> DYKDDDDKSHSPHLPRPHSRVPPHPSSERRAVYIGALFPMSGGWPGGQACQPAVEMALEDVNSRRDILPDYELKLIHHDSKCDPGQATKYLYELLYNDPIKIILMPGCSSVSTLVAEAARMWNLIVLSYGSSSPALSNRQRFPTFFRTHPSATLHNPTRVKLFEKWGWKKIATIQQTTEVFTSTLDDLEERVKEAGIEITFRQSFFSDPAVPVKNLKRQDARIIVGLFYETEARKVFCEVYKERLFGKKYVWFLIGWYADNWFKIYDPSINCTVDEMTEAVEGHITTEIVMLNPANTRSISNMTSQEFVEKLTKRLKRHPEETGGFQEAPLAYDAIWALALALNKTSGGGGRSGVRLEDFNYNNQTITDQIYRAMNSSSFEGVSGHVVFDASGSRMAWTLIEQLQGGSYKKIGYYDSTKDDLSWSKTDKWIGGSPPADQTLVIKTFRFLSQKLFISVSVLSSLGIVLAVVCLSFNIYNSHVRYIQNSQPNLNNLTAVGCSLALAAVFPLGLDGYHIGRNQFPFVCQARLWLLGLGFSLGYGSMFTKIWWVHTVFTKKEEKKEWRKTLEPWK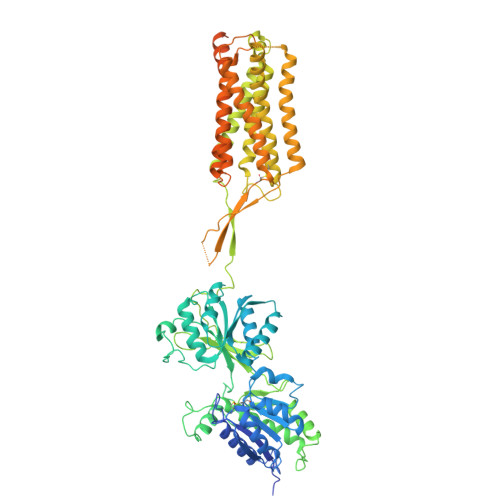LYATVGLLVGMDVLTLAIWQIVDPLHRTIETFAKEEPKEDIDVSILPQLEHCSSRKMNTWLGIFYGYKGLLLLLGIFLAYETKSVSTEKINDHRAVGMAIYNVAVLCLITAPVTMILSSQQDAAFAFASLAIVFSSYITLVVLFVPKMRRLITRGEWQSEAQDTMKTGSSTNNNEEEKSRLLEKENRELEKIIAEKEERVSELRHQLQSRQQLRSRRHPPTPPEPSGGLPRGPPEPPDRLSCDGSRVHLLYKHHHHHH> MVDGNYSVASNVMVPMRDGVRLAVDLYRPDADGPVPVLLVRNPYDKFDVFLWSTQSTNWLEFVRDGYAVVIQDTRGLFASEGEFVPHVDDEADAEDTLSWILEQAWCDGNVGMFGKAYLGVTQWQAAVSGVGGLKAIAPSMASADLYRAPWYGPGGALSVEALLGWSALIGRQLITSRSDARPEDAADFVQLAAILNDVAGAASVTPL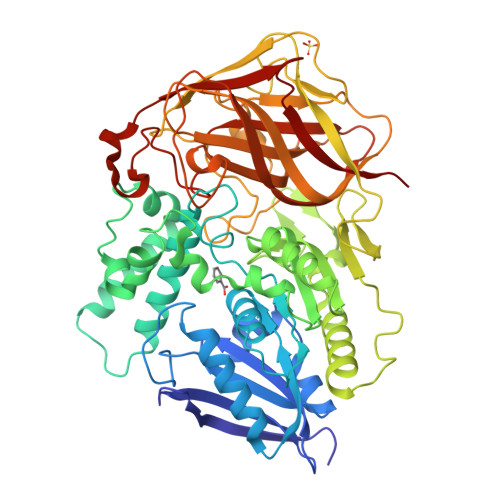AEQPLLGRLIPWVIDQVVDHPDNDESWQSISLFERLGGLATPALITAGWYDGFVGESLRTFVAVKDNADARLVVGPWSHSNLTGRNADRKFGIAATYPIQEATTMHKAFFDRHLRGETDALAGVPKVRLFVMGIDEWRDETDWPLPDTAYTPFYLGGSGAANTSTGGGTLSTSISGTESADTYLYDPADPVPSLGGTLLFHNGDNGPADQRPIHDRDDVLCYSTEVLTDPVEVTGTVSARLFVSSSAVDTDFTAKLVDVFPDGRAIALCDGIVRMRYRETLVNPTLIEAGEIYEVAIDMLATSNVFLPGHRIMVQVSSSNFPKYDRNSNTGGVIAREQLEEMCTAVNRIHRGPEHPSHIVLPIIKR> MNGIHDVGGMDGFGKVMYVKEEEDIYFTHDWERLAFGLVAGCKAQGLGMKAFDEFRIGIELMRPVDYLTSSYYGHWIATVAYNLVDTGVLDEKELDERTEVFLKKPDTKIPRREDPALVKLVEKALYDGLSPLREISASPRFKVGERIKAKNIHPTGHTRFPRYARDKYGVIDEVYGAHVFPDDAAHRKGENPQYLYRVRFEAEELWGYKQKDSVY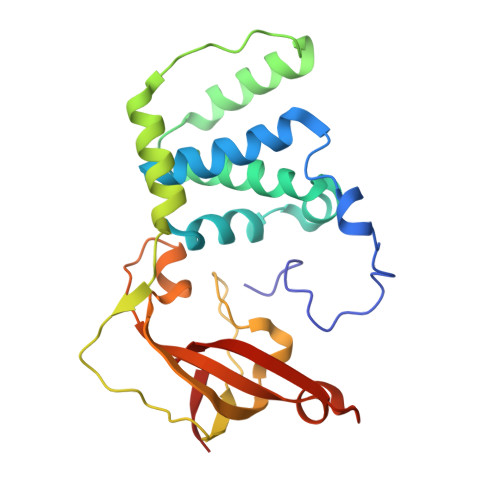IDLWESYMEPVSH>GSPSRSPEFFYWRAKSQMCEVKGWVPTHRGFPWGPELPGDLILSRRAYVSCDLTSCFKFFIAYGLSANQHLLNTSMEWEESLYKTPIGSASTLSTSEMILPGRSSSACFDGLKWTVLVANGRDRNSFIMIKYGEEVTDTFSASRGGPLRLPNSECICIEGSCFVIVSDGPNVNQSVHRIYELQNGTVQRWKQLNTTGINFEYSTCYTINNLIKCTGTNLWNDAKRPLLRFTKELNYQIVEPCNGAPTDFPRGGLTTPSCKMAQEKGEGGIQGFILDEKPAWTSKTKAESSQNGFVLEQI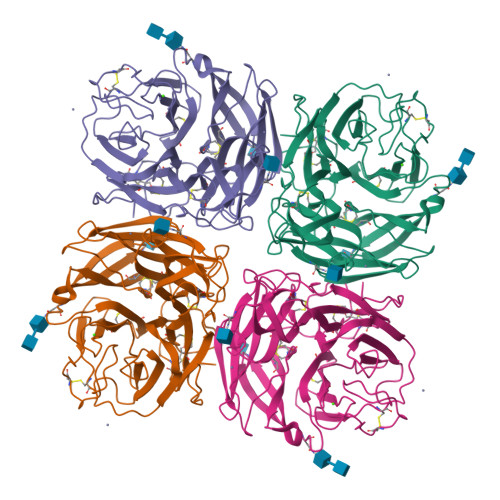PNGIESEGTVSLSYELFSNKRTGRSGFFQPKGDLISGCQRICFWLEIEDQTVGLGMIQELSTFCGINSPVQNINWDS[2x]> FSDXSSVPNF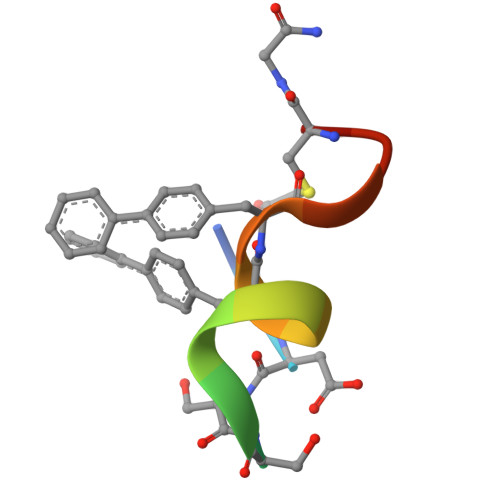FRNCX> MLESK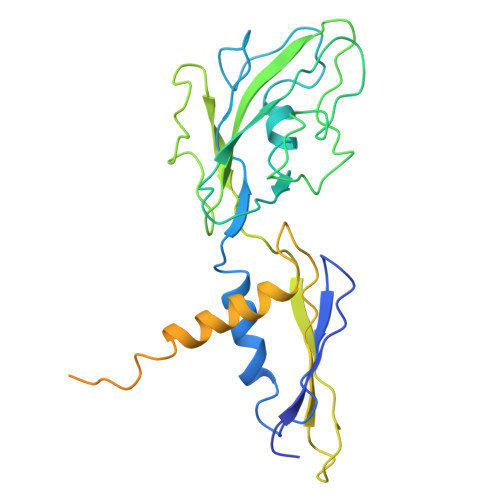LKAPVFTATTQGDHYGEFVLEPLERGFGVTLGNPLRRILLSSIPGTAVTSVYIEDVLHEFSTIPGVKEDVVEIILNLKELVVRFLDPKMASTTLILRAEGPKEVRAGDFTPSADVEIMNPDLHIATLEEGGKLYMEVRVDRGVGYVPAERHGIKDRINAIPVDAIFSPVRRVAFQVEDTRLGQRTDLDKLTLRIWTDGSVTPLEALNQAVAILKEHLNYFANPEASLLPTPEVSKGEKRESAEEDLDLPLEELGLSTRVLHSLKEEGIESVRALLALNLKDLRNIPGIGERSLEEIRQALAKKGFTLKE>MEQEKVQELVSQMTLDEKIAQCLQLSPFLFKGTNKNAELTGPLLQEMKLTDAHTENAGSVLGSSSALDMIGIQEAYLKTNRLGIPLVFMADVIHGYKTVFPIPLALGCSFDRETVRVMAEVSALEATADGHHVTFSPMLDLVRDPRWGRVMESTGEDPFLNSELGKAMVDGYQGDASKLNENLEQMAACVKHFAAYGAAEAGLEYNTVNMSTRELYQNYLPAYNAAIQAGAKLVMTAFNVVDGIPATMNKWLNRDVLRGEMEFDGVLISDWGAVAEVINHGTARNPKEAAQFSMEAGVDLEMMTTCYIHELKGLIEEGKLSENLLDEAVLRMLNLKNDLGLFEDPYRGLKNNDRTKDILTDESRGKARAAGVESAVLLENKSRLLPLAKEAKIALVGPLATSPDILGGWNVYGEEKDGINVETGLREVFETVEVVSTEYTELSEEDKVAVKAAVQNMDVVVLALGEKNEWGGEAGSLATIRLPEAQYQLAKFVQTLGKPVVITLFNGRPLEVKELAESSDALLELWFPGTEAGRVTADLLSGASNPSGKLSMSFPQTTGQIPVYYNHLRTGRPQTPENKGERYVSHYLDIPNEPFYPFGYGKSYSEFELKTSSLPKELNLGESLHVEVTIKNISDIAGKEVIQVYLQDVTASISRPVKELKAFEKVALQAGEEKTVTFELTSEAFSFYNHQLEKVQEPGLHRVFVGTSSEDVDVFEVEVGGYVLEHHHHHH[2x]

In the gene cluster containing the lin1839 gene, the lin1840 gene encodes a putative glycoside hydrolase family (GH) 3 β-glucosidase (BGL) (GenBank accession number: CAC97071.1). The structure showed that Lin1840r forms a dimer of identical subunits each composed of three domains. The active center of Lin1840r is located at the interface of domains 1 and 2 as in the cases of known GH3 BGLs.

To clarify the binding modes of inhibitors, Lin1840r-inhibitor complex structures were determined. Three glucosidase inhibitors, GDL, IFG, and DNJ, consistently exhibited competitive-type inhibition with Ki values of less than 1 mM. IFG showed the strongest inhibition among all the inhibitors examined, the Ki value being 4.1 μM. In complex structures with IFG and GDL, which are Glc analogs, the ligands are located at the same position as Glc, suggesting that IFG and GDL compete with substrates for subsite −1. In the case of the IFG complex structure, on the other hand, an unwound helix (amino acids 36–47) in domain 1 is inserted between the aromatic rings of Tyr583 and Trp271. Thr40 in this loop forms a hydrogen bond with the 6-OH group of IFG. This loop might be involved in substrate binding in solution.> GSTPDQQTLLHFIMDSYNKQRMPQEITNKILKEEFSAEENFLILTEMATNHVQVLVEFTKKLPGFQTLDHEDQIALLKGSAVEAMFLR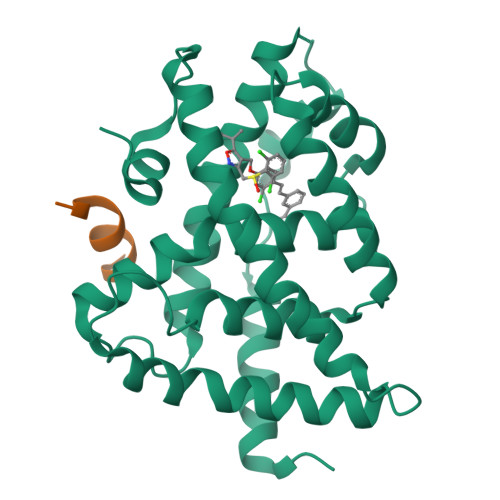SAEIFNKKLPSGHSDLLEERIRNSGISDEYITPMFSFYKSIGELKMTQEEYALLTAIVILSPDRQYIKDREAVEKLQEPLLDVLQKLCKIHQPENPQHFAELLGRLTELRTFNHHHAEMLMSWRVNDHKFTPLLEEIWDVQ;> AHQLLRYLLDA> ARAAFLFKTVGFGGLQNVPINDELSSHLLRAGNSPWQLTQFLDWISLGRGLATSALVPTAGSRYYQMSCLLSGTLQIPFRPNHRWGDIRFLRLVWSAPTLDGLVVAPPQVLAQPALQAQADRVYDCDDYPFLARDPRFKHRVYQQLSAVTLLNLTGFGPISYVRVDEDMWSGDVNQLLMNYFGHTFAEIAYTLCQASANRPWEHDGTYARMTQIILSLFWLSYVGVI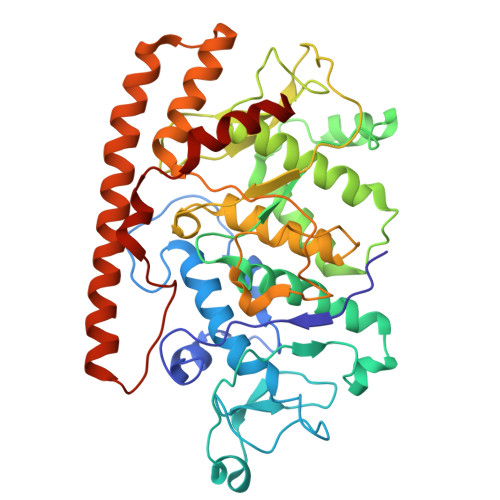HQQNTYRTFYFQCNRRGDAAEVWILSCSLNHSAQIRPGNRSLFVMPTSPDWNMDVNLILSSTLTGCLCSGSQLPLIDNNSVPAVSRNIHGWTGRAGNQLHGFQVRRMVTEFCDRLRRDGVMTQAQQNQIEALADQTQQFKRDKLEAWAREDDQYNQANPNSTMFRTKPFTNAQWGRGNTGATSAAIAALI> GSPELRQEHQQLAQEFQQLLQEIQQLGRELLKGELQGIKQLREASEKARNPEKKSVLQKILEDEEKHIELLETLQQTGQEAQQLLQELQQTGQELWQLGGSGGP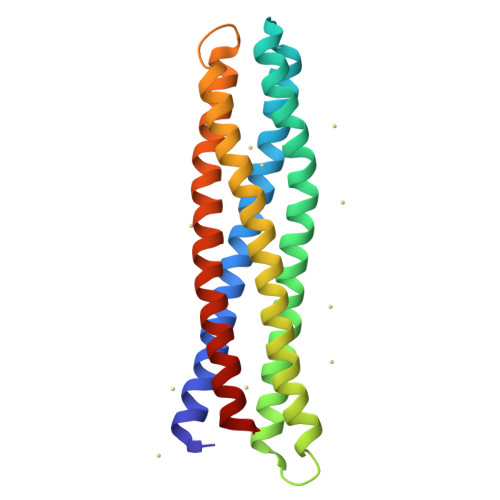ELRQKHQQLAQKIQQLLQKHQQLGAKILEDEEKHIELLETILGGSGGDELRELLKGELQGIKQYRELQQLGQKAQQLVQKLQQTGQKLWQLG>[2x]MTSNLIKFDDQNKVFHLHNKQISYLLSIEDGGTLSHLYF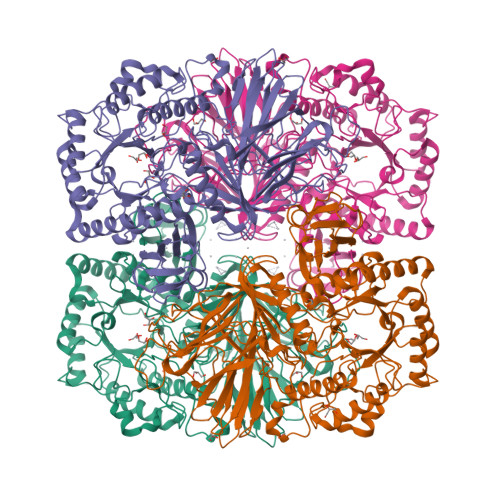GGAVKNYNNQLKYPRLDRGFSGNLPESLDRTFSRDSLPKEYSSAGEMDFHTPATIVRNPDGSNALFLAYKSYKIEDGKPDLKGLPHSWTKEDDEAQTLIVTLEDKVSKLEYDLLYTIYRDRPVIVRSVQVHNHGEEAVYLEKVASMQMDYVDKDFEVITLPGAHANERRVQRENIGQGIKVFSSYRGTSSHQMNPFMALVDHDTNEFMGEAYGFALAYSGNHKFEVERDQFGQIHVNTGINDYNFKWKLNPNEEFQTPEVLMVYSDQGLNKMSQAFHSLIHERIMRSKFKDQIRPVLVNNWEATYFDFNEDKLKTIVDKAKKLGLEMFVLDDGWFGHRDDDNSSLGDWKVYKKKFPNGLGHFADYVHEQGLKFGLWFEPEMISYESNLYKEHPDYLMHVPGRKPCPSRNQYVLELGRKEVRDNIFEQMVKILDSKKIDYIKWDMNRSLSDIYESDLPADQQGEAYHRYVLGYYDLLNKLVTRYPDILFEGCSGGGGRFDVGQAYYTPQIWASDNTDAIERLKIQYGTSLVYPQSMMTSHVSVSPNEQNGRITPFNTRGAVAMWGDLGYELDLTKMSDEESDQVVKQVTEYKKIREVTQFGTLYRLKASASNQCAWMMVDSNKNEAVVTVVNVMAHAQPYCTKTKLAGLDPDKRYKNLETDEVFGGDELMHLGFYDPIERGDFKAKMYHFKAIN> LPQTVRIGTATTYAPFSSKDAKGEFIGFDIDLGNEMCKRMQVKCTWVASDFDALIPSLKAKKIDAIISSLSITDKRQQEIAFSDKLYAADSRLIAAKGSPIQPTLESLKGKHVGVLQGSTQEAYANDNWRTKGVDVVAYANQDLIYSDLTAGRLDAALQDEVAASEGFLKQPAGKEYAFAGPSVKDKKYFGD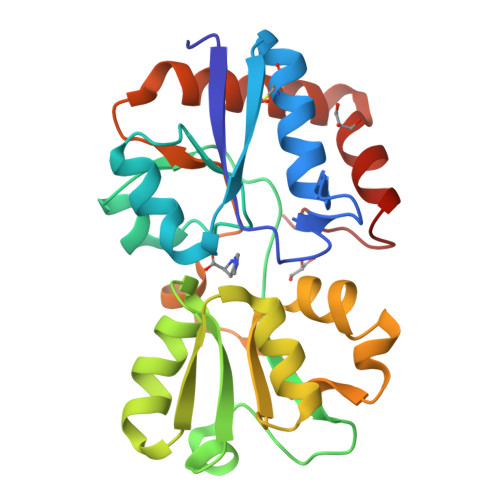GTGVGLRKDDTELKAAFDKALTELRQDGTYDKMAKKYFDFNVYGD>MGHHHHHHHHHHSSGHIEGRHMKRHYEAVVIGGGIIGSAIAYYLAKENKNTALFESGTMGGRTTSAAAGMLGAHAECEERDAFFDFAMHSQRLYKGLGEELYALSGVDIRQHNGGMFKLAFSEEDVLQLRQMDDLDSVSWYSKEEVLEKEPYASGDIFGASFIQDDVHVEPYFVCKAYVKAAKMLGAEIFEHTPVLHVERDGEALFIKTPSGDVWANHVVVASGVWSGMFFKQLGLNNAFLPVKGECLSVWNDDIPLTKTLYHDHCYIVPRKSGRLVVGATMKPGDWSETPDLGGLESVMKKAKTMLPPIQNMKVDRFWAGLRPGTKDGKPYIGRHPEDSRILFAAGHFRNGILLAPATG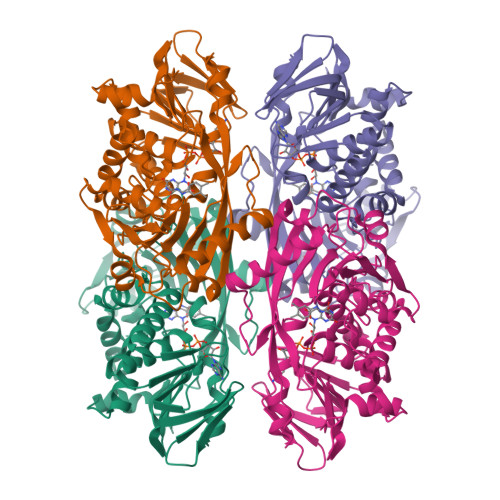ALISDLIMNKEVNQDWLHAFRIDRKEAVQI[2x]2-[(2-acetylphenyl)sulfanyl]benzoic 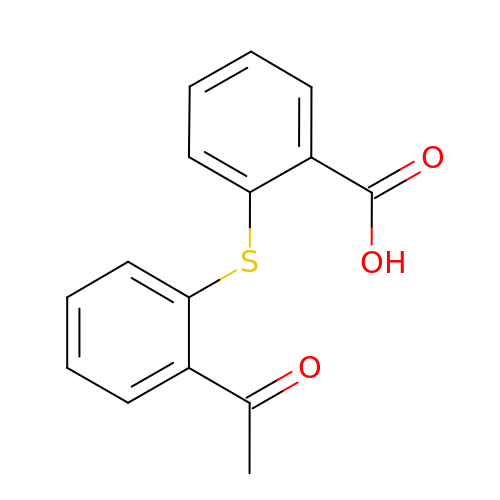acid | C15 H12 O3 S | UVKUNTVZWDIEDN-UHFFFAOYSA-N The CysN polypeptide also contains a C-terminal APS (adenosine-5’-phosphosulfate) kinase domain (CysC), which exists as a separate enzyme in other bacteria and plants. Alternatively, APS can be phosphorylated at the 3′-position by APS kinase (CysC) to generate 3′-phosphoadenosine 5′-phosphosulfate (PAPS), a substrate for sulfotransferases that catalyze the transfer of the sulfate group onto a variety of metabolites. The structure of CysC is characterized by the canonical α/β-purine nucleotide binding fold, consisting of a five-stranded parallel β-sheet which is flanked on both sides by two α-helices. Structural features typical of APS kinases of this fold family, including the P-loop required for ATP binding (residues 452–458 in CysC), the conserved LDGD motif (residues 477–480) and the lid region (residues 552–581) above the P-loop which closes upon substrate binding, are also found in CysC.

CysC contains three cysteine residues, Cys514, Cys549 and Cys556, and we therefore examined their role in CysC activation. The Cys556Ala mutant also displayed activation upon addition of DTT, but to a lesser extent. Surprisingly amino acid replacement at position 556 resulted in mutants with severely impaired catalytic activity. The Cys556Ala mutant showed little activity upon treatment with DTT, whereas the conservative replacement of Cys556 by serine resulted in complete loss of enzymatic activity, which could not be rescued by the addition of DTT. Overall, the crystal structure of this mutant shows little alteration compared to the wild-type, as indicated by the r.m.s.d. of 0.5 Å over 143 equivalent Cα atoms after superposition with the crystal structure of the binary complex of wild-type enzyme. The crystals of the mutant were obtained under the same conditions as those of the wild-type CysC•ADP complex, however no bound ADP was observed in any of the subunits. During structure refinement it became evident that an approximately 30 residue long segment (residues 552–581) in both chains of the asymmetric unit lack electron density and cannot be modeled, possibly due to loop disorder. This peptide stretch corresponds to the lid domain that closes over the active site cleft upon binding of the nucleotide ADP or AMP-PNP, respectively. The mutagenesis results highlighted the role of Cys556 as an essential residue in proper function of the lid region of the enzyme. Lid closure is essential to enzymatic activity and disturbance of the packing interactions of the lid with the protein core, even by a conservative cysteine to serine substitution, leads to the loss of enzymatic activity.

>GSHMSPNTVRHRSLVTAQDRPPRGKTVWFTGLSGSGKSSVAMLVERKLLEKGISAYVLDGDNLRHGLNADLGFSMADRAENLRRLSHVATLLADCGHLVLVPAISPLAEHRALARKVHADAGIDFFEVFCDTPLQDSERRDPKGLYAKARAGEITHFTGIDSPYQRPKNPDLRLTPDRSIDEQAQEVIDLLES[2x]> GSVGPKTGEENQVLVPNLNPTPENLEVVGDGFKITSSINLVGEEEADENAVNALREFLTANNIEINSENDPNSTTLIIGEVDDDIPELDEALNGTTAENLKEEGYALVSNDGKIAIEGKDGDGTFYGVQTFKQLVKESNIPEVNITDYPTVSARGIVEGFYGTPWTHQDRLDQIKFYGENKLNTYIYAPKDDPYHREKWREPYPESEMQRMQELINASAENKVDFVFGISPGIDIRFDGDAGEEDFNHLITKAESLYDMGVRSFAIYWDNIQDKSAAKHAQVLNRFNEEFVKAKGDVKPLITVPTEYDTGAMVSNGQPRAYTRIFAETVDPSIEVMWTGPGVVTNEIPLSDAQLISGIYDRNMAVWWNYPVTDYFKGKLALGPMHGLDKGLNQYVDFFTVNPMEHAELSKISIHTAADYSWNMDNYDYDKAWNRAIDMLYGDLAEDMKVFANHSTRMDNKTWAKSGREDAPELRAKMDELWNKLSSKEDASALIEELYGEFARMEEACNNLKANLPEVALEECSRQLDELITLAQGDKASLDMIVAQLNEDTEAYESAKEIAQNKLNTALSSFAVISEKVAQSFIQEALS;> VAHSGAK

Reversible protein O-GlcNAcylation is achieved by the action of two enzymes, O-GlcNAc transferase (OGT) and O-GlcNAcase (OGA). Although it is unclear whether CpOGA is a physiological OGA, it shows significant in vitro O-GlcNAcase activity on O-GlcNAc proteins in lysates from human cell lines and possesses a putative substrate-binding groove conserved with hOGA (Rao et al., 2006; Schimpl et al., 2010). We report the molecular details of the interaction of a bacterial O-GlcNAcase homolog with three different synthetic glycopeptides derived from characterized O-GlcNAc sites in the human proteome. In addition to extensive contacts with the sugar, O-GlcNAcase recognizes the peptide backbone through hydrophobic interactions and intramolecular hydrogen bonds, while avoiding interactions with the glycopeptide side chains.

Here we report that CpOGA, like hOGA (Schimpl et al., 2010), possesses activity toward synthetic glycopeptides derived from validated O-GlcNAc sites in the human proteome, namely p53 (Ser149 [Yang et al., 2006]), TAK1-binding protein 1 (TAB1, Ser395 [Schimpl et al., 2010]), and hOGA itself (Ser405 [Lazarus et al., 2006]). To investigate the molecular basis of this substrate specificity, we exploited the catalytic acid mutant of CpOGA, D298N, which is inactive yet unaffected in its ability to bind substrate (Rao et al., 2006). We generated an alternative CpOGA crystal form with a highly accessible active site and determined the structures of CpOGA D298N in complex with the p53-, TAB1-, and hOGA-derived O-GlcNAc peptides. The O-GlcNAc sugar occupies the same position in all three structures (maximum atomic shift of 0.2 Å). Strikingly, the backbones of all three glycopeptides run in the same direction, together defining the −4 through +3 subsites, and adopt similar conformations near the O-GlcNAc site (maximum Cα shift of 1.8 Å for the −2 to +1 subsites). Hydrophobic stacking of the solvent-exposed Tyr189 (Tyr69 in hOGA) aromatic side chain with the −1 and −2 peptide bonds contributes a major amount (∼30% of the buried surface) of the interaction between the enzyme and the peptide component of the glycopeptides. All three glycopeptides adopt a “V-shaped” conformation that allows the sugar to penetrate the OGA active site. Interestingly, for two of the peptides, this conformation appears to be stabilized by intramolecular hydrogen bonds. The hOGA-derived glycopeptide forms a hydrogen bond between the histidine in the −1 subsite and the backbone carbonyl oxygen of the O-GlcNAc serine. For the p53-derived glycopeptide, a hydrogen bond is observed between the aspartic acid in the −1 subsite and the threonine in the +1 subsite. Such intramolecular interactions may stabilize the OGA-bound conformation of these glycopeptides, explaining the significantly lower Kms compared to the TAB1-derived peptide.> MAYFDYTSAKPVDERILEAMLPYMTESFGNPSSVHSYGFKAREAVQEAREKVAKLVNGGGGTVVFTSGATEANNLAIIGYAMRNARKGKHILVSAVEHMSVINPAKFLQKQGFEVEYIPVGKYGEVDVSFIDQKLRDDTILVSVQHANNEIGTIQPVEEISEVLAGKAALHIDATASVGQIEVDVEKIGADMLTISSNDIYGPKGVGALWIRKEAKLQPV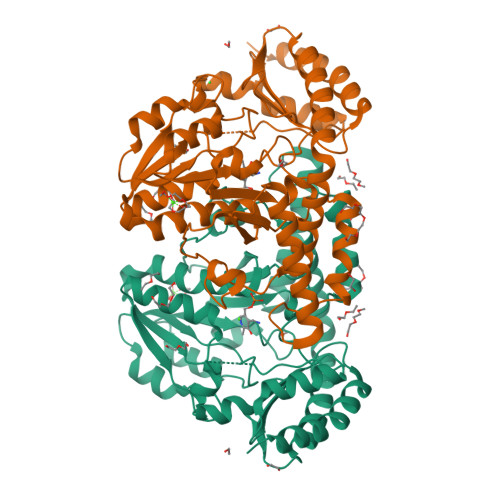ILGGGQENGLRSGSENVPSIVGFGKAAEITAMEWREEAERLRRLRDRIIDNVLKIEESYLNGHPEKRLPNNVNVRFSYIEGESIVLSLDMAGIQASTGSACSSKTLQPSHVLMACGLKHEEAHGTLLLTLGRYNTDEDVDRLLEVLPGVIERLRSMSPLYRR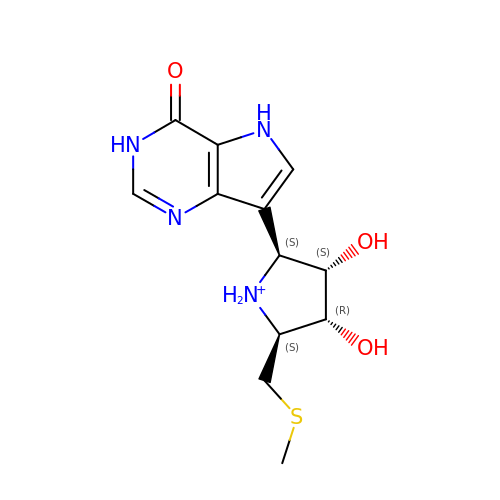3,4-DIHYDROXY-2-[(METHYLSULFANYL)METHYL]-5-(4-OXO-4,5-DIHYDRO-3H-PYRROLO[3,2-D]PYRIMIDIN-7-YL)PYRROLIDINIUM | C12 H17 N4 O3 S | CEGIKIXYDFDYDN-RXDXJJGDSA-O>[5x]MRYIDDELENQTILITGGAGFVGSNLAFHFQENHPKAKVVVLDKFRSNTLFSNNRPSSLGHFKNLIGFKGEVIAADINNPLDLRRLEKLHFDYLFHQAAVSDTTMLNQELVMKTNYQAFLNLLEIARSKKAKVIYASSAGVYGNTKAPNVVGKNESPENVYGFSKLCM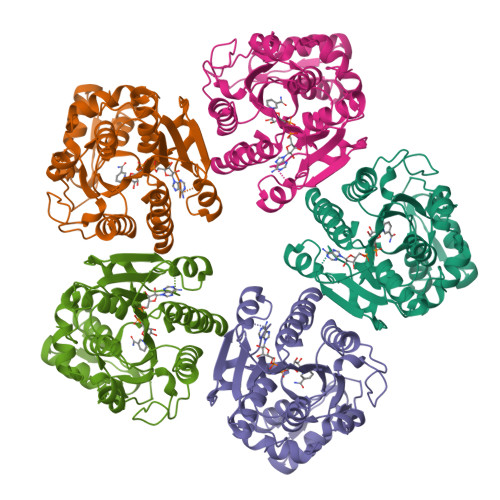DEFVLSHSNDNVQVGLRYFNVYGPREFYKEKTASMVLQLALGAMAFKEVKLFEFGEQLRDFVYIEDVIQANVKAMKAQKSGVYNVGYSQARSYNEIVSILKEHLGDFKVTYIKNPYAFFQKHTQAHIEPTILDLDYTPLYDLESGIKDYLPHIHAIFKGQRAKGELNSKLEGKPIPNLLGLDSTRTGHHHHHHH2-HYDROXY-5-(2-MERCAPTO-ETHYLSULFAMOYL)-BENZOIC 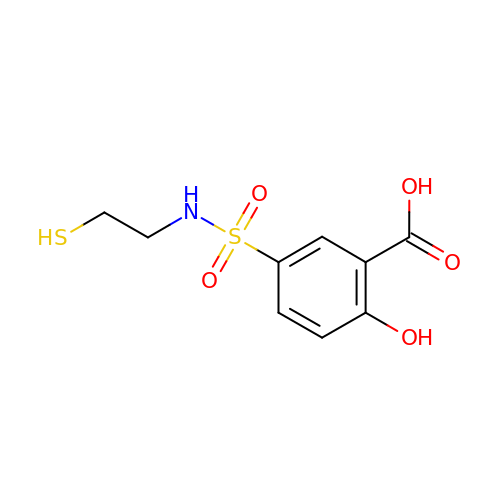ACID | C9 H11 N O5 S2 | UCQUNSCHVXCSCJ-UHFFFAOYSA-N> MRGSHHHHHHGMASNEFFPVVLVINCGSSSIKFSVLDVATCDVLMAGIADGMNTENAFLSINGDKPINLAHSNYEDALKAIAFELEKRDLTDSVALIGHRIGHGGELFTQSVIITDEIIDNIRRVSPLAPLHNYANLSGIDAARHLFPAVRQVAVFDTSFHQTLAPEAYLYGLPWEYFSSLGVRRYGFHGTSHR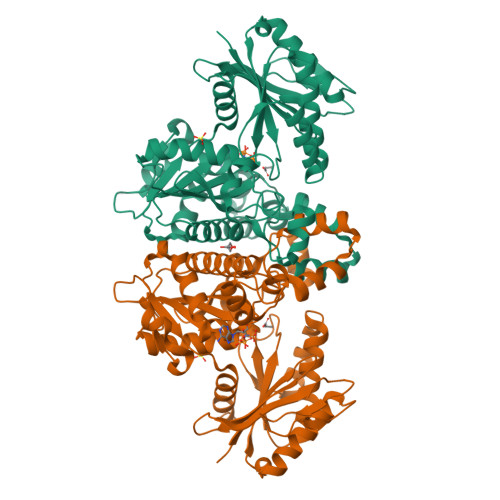YVSRRAYELLDLDEKDSGLIVAHLGNGASICAVRNGQSVDTSMGMTPLEGLMMGTRSGDVDFGAMAWIAKETGQTLSDLERVVNKESGLLGISGLSSDLRVLEKAWHEGHERARLAIKTFVHRIARHIAGHAASLHRLDGIIFTGGIGENSVLIRQLVIEHLGVLGLTLDVEMNKQPNSHGERIISANPSQVICAVIPTNEEKMIALDAIHLGNVKA>[2x]MASGMTVTDA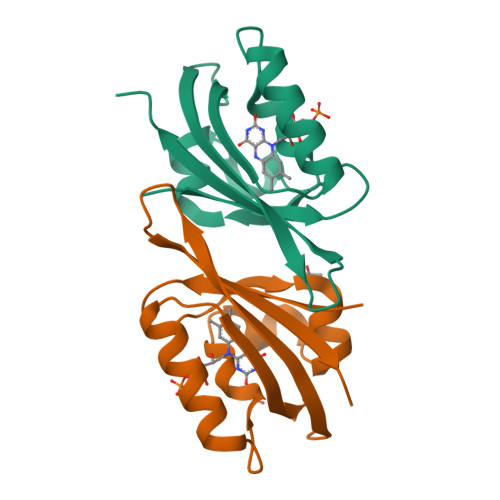GADQPIVFVNRAFSTITGYAPNEVLGRNARFLQGPQTDAATVARLREAIAAARPIQERILNYRKDGQPFWNQLSISPVRDETGNVVAFVGVQTDVTAHHHHHH1,5-anhydro-6-O-phosphono-D-glucitol | C6 H13 O8 P | 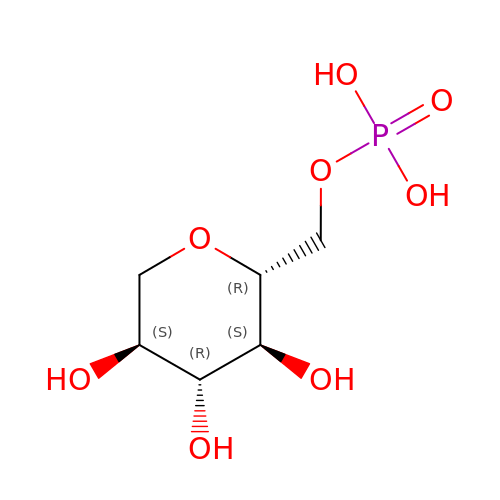KAJAXXUCVJFKFM-SLPGGIOYSA-N>MRQVAIYGKGGIGKSTTTQNLTSGLHAMGKTIMVVGCDPKADSTRLLLGGLAQKSVLDTLREEGEDVELDSILKEGYGGIRCVESGGPEPGVGCAGRGIITSINMLEQLGAYTDDLDYVFYDVLGDVVCGGFAMPIREGKAQEIYIVASGEMMAL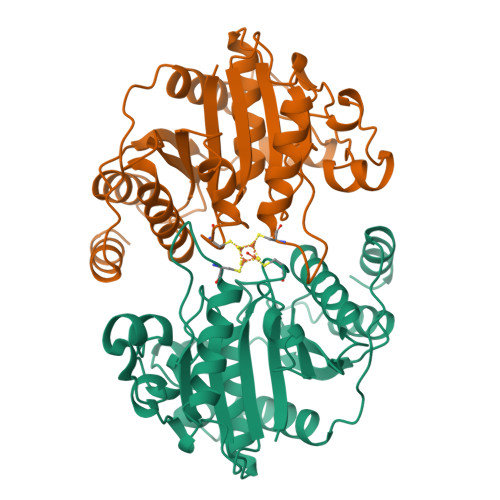YAANNISKGIQKYAKSGGVRLGGIICNSRKVANEYELLDAFAKELGSQLIHFVPRSPMVTKAEINKQTVIEYDPTCEQAEEYRELARKVDANELFVIPKPMTQERLEEILMQYG[2x]> DPGCLPDWSSYKGHCYKVFKKVGTWEDAEKFCVENSGHLASIDSKEEADFVTKLASQTLTKFVYDAWIGLRDESKTQQCSPQWTDGSSVVYENVDEPTKCFGLDVHTEYRTWTDLPCGEKNPFICKSRLPH;> DEGCLPDWSSYKGHCYKVFKVEKTWADAEKFCKELVNGGHLMSVNSREEGEFISKLA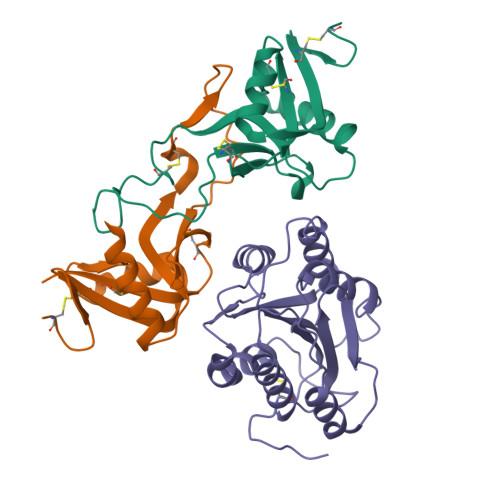LEKMRIVLVWIGLSHFWRICPLRWTDGARLDYRALSDEPICFVAESFHNKWIQWTCNRKKSFVCKYRV;> EDISEPPLHDFYCSRLLDLVFLLDGSSRLSEAEFEVLKAFVVDMMERLRISQKWVRVAVVEYHDGSHAYIGLKDRKRPSELRRIASQVKYAGSQVASTSEVLKYTLFQIFSKIDRPEASRIALLLMASQEPQRMSRNFVRYVQGLKKKKVIVIPVGIGPHANLKQIRLIEKQAPENKAFVLSSVDELEQQRDEIVSYLCDLAPEAPPPT> MSRDRFRSRGGGGGGFHRRGGGGGRGGLHDFRSPPPGMGLNQNRGPM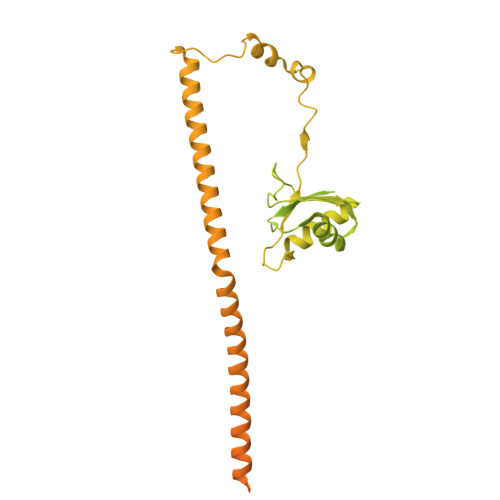GPGPGGPKPPIPPPPPHQQQPQQPPPQQPPPQQPPPHQQPPPHQPPHQQPPPPPQDSSKPVVPQGPGSAPGVSPAPPPAGSAPPANPPTTGAPPGPGPTPTPPPAVTSATPGPPPPSTPSSGVSTTPPQSGGPPPPPAGGAGPGPKQGPGPGPGGPKGGKMPGGPKPGGGPGMGAPGGHPKPPHRGGGEPRGGRQHHPPYHQQHHQGPPPGGPAARTEEKISDSEGFKANLSLLRRPGEKTYTQRCRLFVGNLPADITEDEFKRLFAKYGEPGEVFINKGKGFGFIKLESRALAEIAKAELDDTPMRGRQLRVRFATHAAALSVRNLSPYVSNELLEEAFSQFGPIERAVVIVDDRGRSTGKGIVEFASKPAARKAFERCSEGVFLLTTTPRPVIVEPLEQLDDEDGLPEKLAQKNPMYQKERETPPRFAQHGTFEYEYSQRWKSLDEMEKQQREQVEKNMKDAKDKLESEMEDAYHEHQANLLRQDLMRRQEELRRMEELHSQEMQKRKEMQLRQEEERRRREEEMMIRQREMEEQMRRQREESYSRMGYMDPRERDMRMGGGGTMNMGDPYGSGGQKFPPLGGGGGIGYEANPGVPPATMSGSMMGSDMRTERFGQGGAGPVGGQGPRGMGPGTPAGYGRGREEYEGPNKKPRF>[4x]SNADSSNIALPKFESLIKSGITDPTELEKYGVEHYTYEEYAKHIQELKDYAK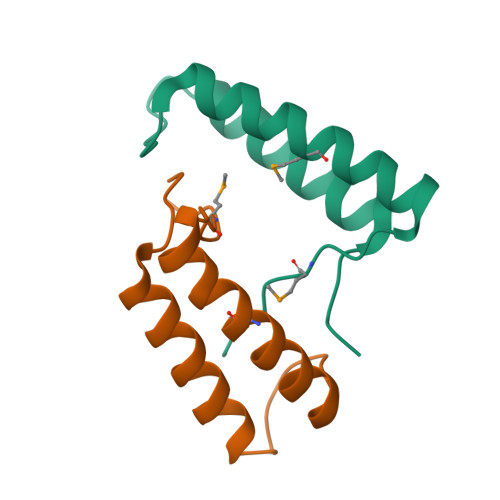DPNAVKDVSQKDLEETIKKMEQELEKIKTEGLKIMKPITIENEDGSQISIAYNYAAID The circadian clock of the cyanobacterium Synechococcus elongatus can be reconstituted in vitro by three proteins, KaiA, KaiB and KaiC. Homo-hexameric KaiC displays kinase, phosphatase and ATPase activities; KaiA enhances KaiC phosphorylation and KaiB antagonizes KaiA. The crystal structure of KaiC from S. elongatus revealed a hexamer in the shape of a double doughnut with approximate dimensions 100×100 Å, whereby the N-terminal CI and C-terminal CII halves of subunits are joined by a 15-amino acid linker. Two phosphorylation sites (P-sites), T432 and S431 that are both located in the CII half were identified in KaiC.

To analyze the phosphorylation patterns of KaiC P-site mutants and to visualize potential conformational variations in the vicinity of bound ATP and residues 432 and 431 at hexamer subunit interfaces, we determined crystal structures of the S. elongatus KaiC single mutants T432A (TSa), S431A (TaT), S431D (TdT), and T426N (nST) and the double mutants T426A/T432A (aSa) and S431A/T432E (Tae). b KaiC mutations xyz or mutants KaiCxyz are sequentially shown in order of sites x = 426, y = 431, and z = 432 where the wild-type residue is in upper case and mutated residues are shown in lower case, i.e. Tsa or KaiCTSa, where the residue at position 426 is T, the residue at position 431 is S, and the residue at position 432 is mutated to A. The structures of the TdT, nST and aSa mutants provide further support for the conclusion that T432 is the principal phosphorylation site because it lies closest to the γ-phosphate. Moreover, the hampered ability of KaiB to antagonize KaiA with the KaiCaST and KaiCnST mutants could be due to their altered electrostatic surface potentials relative to wt-KaiC as a result of the lack of a phosphorylatable residue at position 426. The combined structural data expose subtle changes in the orientations of the H423-I433 loop region harboring phosphorylated residues relative to the γ-phosphate of ATP compared with the structure of wt-KaiC.

>MTSAEMTSPNNNSEHQAIAKMRTMIEGFDDISHGGLPIGRSTLVSGTSGTGKTLFSIQFLYNGIIEFDEPGVFVTFEETPQDIIKNARSFGWDLAKLVDEGKLFILDASPDPEGQEVVGGFDLSALIERINYAIQKYRARRVSIDSVTSVFQQYDASSVVRRELFRLVARLKQIGATTVMTTERIEEYGPIARYGVEEFVSDNVVILRNVLEGERRRRTLEILKLRGTSHMKGEYPFTITDHGINIFPLGAMRLTQRSSNVRVSSGVVRLDEMCGGGFFKDSIILATGATGTGKTLLVSRFVENACANKERAILFAYEESRAQLLRNAYSWGMDFEEMERQNLLKIVCAYPESAGLEDHLQIIKSEINDFKPARIAIDSLSALARGVSNNAFRQFVIGVTGYAKQEEITGLFTNTSDQFMGAHSINDSHISTITDTIILLQYVEIRGEMSRAINVFKMRGSWHDKAIREFMISDKGPDIKDSFRNFERIISGSPTRITVDEKSELSRIVRGVQEKGPES[6x]>MNHETFLKRAVTLACEGVNAGIGGPFGAVIVKDGAIIAEGQNNVTTSNDPTAHAEVTAIRKACKVLGAYQLDDCILYTSCEPCPMCLGAIYWARPKAVFYAAEHTDAAEAGFDD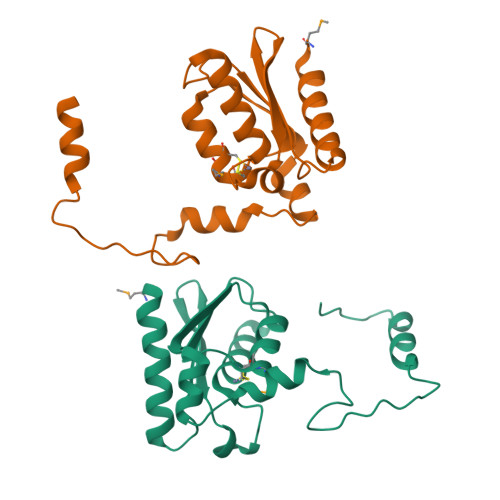SFIYKEIDKPAEERTIPFYQVTLTEHLSPFQAWRNFANKKEYLEHHHHHH[2x]>GSHMSEREKRVSNAVEFLLDSRVRRTPTS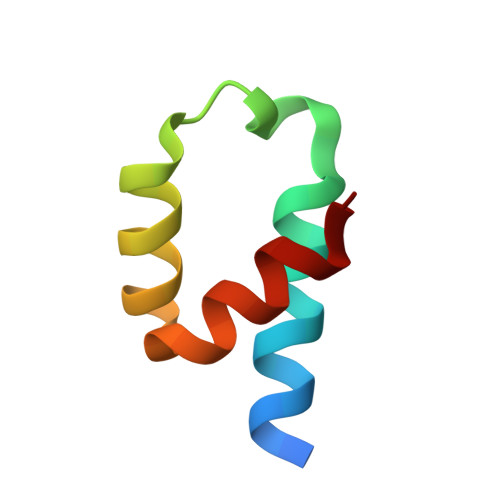SKVHFLKSKGLSAEEICEAFTKVG[5x]> GHMDYLFKLLLIGD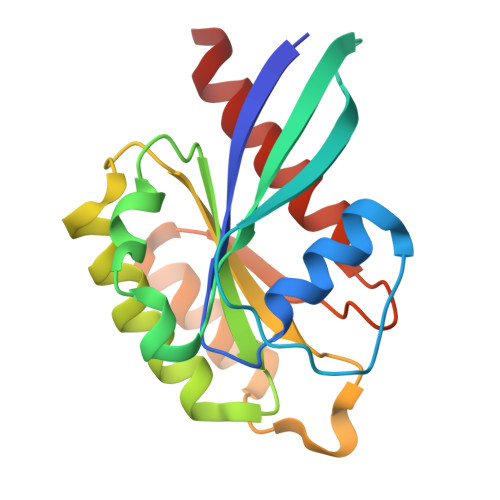SGVGKTCVLFRFSEDAFNSTFISTIGIDFKIRTIELDGKRIKLQIWDTAGQERFRTITTAYYRGAMGIMLVYDITNEKSFDNIRNWIRNIEEHASADVEKMILGNKCDVNDKRQVSKERGEKLALDYGIKFMETSAKANINVENAFFTLARDIKAKMDKK> ACGGACAGAGTGCAC;> CACACCGT;> GAGTGCACTCTGT;> CTTGT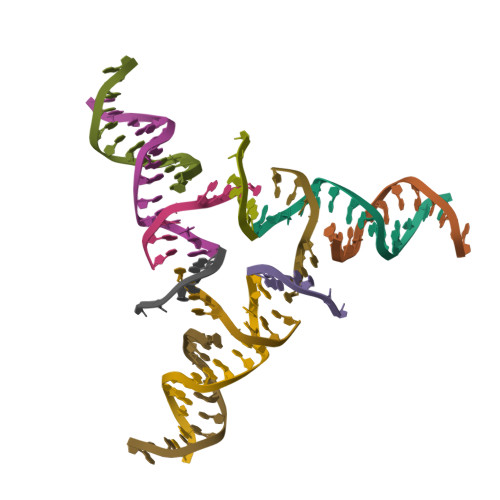G> MSEIGTGFPFDPHYVEVLGSRMHYVDVGPRDGTPVLFLHGNPTSSYLWRNIIPHVAPSHRCIAPDLIGMGKSDKPDLDYRFDDHVRYLDAFIEALG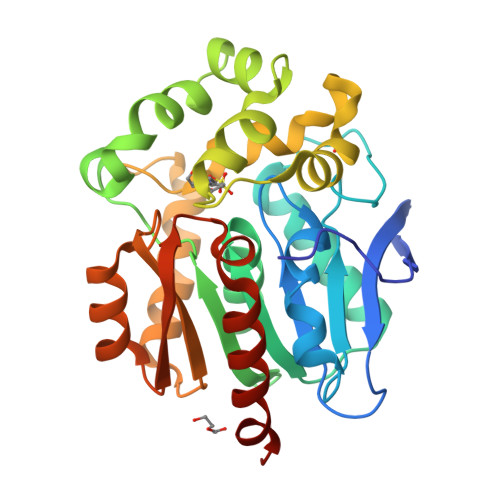LEEVVLVIHDWGSALGFHWAKRNPERVKGIACMEFIRPIPTWDEWPEFARETFQAFRTPDVGRELIIDQNAFIEGALPKCVVRPLTEVEMDHYREPFLKPVDREPLWRFPNELPIAGEPANIVALVEAYMNWLHQSPVPKLLFWGTPGVLIPPAEAARLAESLPNCKTVDIGPGLHYLQEDNPDLIGSEIARWLPALEHHHHHH> SMAATAAEAVASGSGEPREEAGALGPAWDESQLRSYSFPTRPIPRLSQSDPRAEELIENEEPVVLTDTNLVYPALKWDLEYLQENIGNGDFSVYSASTHKFLYYDEKKMANFQNFKPRSNREEMKFHEFVEKLQDIQQRGGE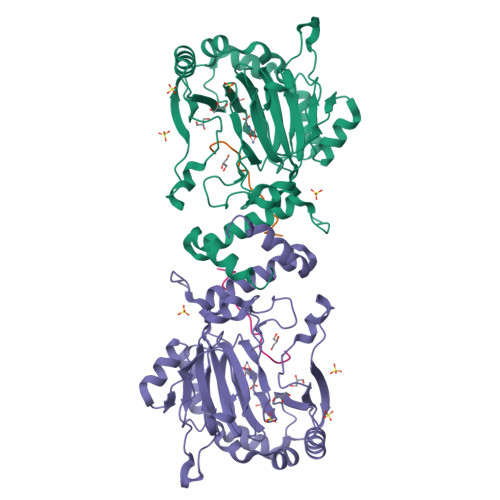ERLYLQQTLNDTVGRKIVMDFLGFNWNWINKQQGKRGWGQLTSNLLLIGMEGNVTPAHYDEQQNFFAQIKGYKRCILFPPDQFECLYPYPVHHPCDRQSQVDFDNPDYERFPNFQNVVGYETVVGPGDVLYIPMYWWHHIESLLNGGITITVNFWYKGAPTPKRIEYPLKAHQKVAIMRNIEKMLGEALGNPQEVGPLLNTMIKGRYN;> GHHHIVKFLLDFGVNVNAADSDG The most frequent PTM reaction catalyzed by FIC enzymes is the addition of AMP using ATP as a cofactor, coined AMPylation or adenylylation. Enterococcus faecalis FIC belongs to class III FIC proteins, which are comprised of a single FIC domain and carry an autoinhibitory glutamate in their C-terminal α-helix. We discover that EfFIC has both AMPylation and deAMPylation activities borne by the same active site. Furthermore, the conserved glutamate implements a Ca2+-controlled metal switch that tunes the balance between these activities without conformational change.

Two crystal structures were obtained by co-crystallization with a non-hydrolyzable ATP analog (ATPγS), for which well-defined electron density was observed for the ADP moiety. To understand how Ca2+ inhibits AMPylation, we determined the crystal structure of EfFICWT-ATPγS-Ca2+. In this structure, Ca2+ is heptacoordinated to the α- and β-phosphates of ATPγS (of which again only the ADP moiety is visible), to the inhibitory glutamate, and to four water molecules. Strikingly, Ca2+ is shifted by 3.2 Å from Mg2+ bound to NmFIC and ATP8. In this position, Ca2+ conflicts with the binding of Mg2+ to ATP, and it cannot interact with the acidic residue from the FIC motif (E115), which is critical for AMPylation. These observations explain why Ca2+ inhibits AMPylation and how it competes with Mg2+. In EfFIC, Ca2+ binds to ATP in a manner that hinders binding of Mg2+ to the canonical AMPylation metal-binding site, thereby inhibiting AMPylation.

>MHHHHHHMLENKLGIINQLELNRVEERVSKENAKRLYDSGDIDRIEVGTFKGLSYIHNYLFEDIYEFAGKVRSQNISKGNFRFAPVMYLEIALEHIDKMPQRNLDEIVAKYVEMNIAHPFREGNGRATRIWLDLILKKELKRVVDWNLINKEDYLSAMERSPVKDLEIKYLISNALTDKINDREIFMKGIDISYYYEGYTEYNVDEL[12x]>[2x]APSFNVDPLEQPAEPSKLAKKLRAEPDMDTSFVGLTGGQIFNEMMSRQNVDTVFGYPGGAILPVYDAIHNSDKFNFVLPKHEQGAGHMAEGYARASGKPGVVLVTSGPGATNVVTPMADAFADGIPMVVFTGQVPTSAIGTDAFQEADVVGISRSCTKWNVMVKSVEELPLRINEAFEIATSGRPGPVLVDLPKDVTAAILRNPIPTKTTLPSNALNQLTSRAQDEFVMQSINKAADLINLAKKPVLYVGAGILNHADGPRLLKELSDRAQIPVTTTLQGLGSFDQEDPKSLDMLGMHGCATANLAVQNADLIIAVGARFDDRVTGNISKFAPEARRAAAEGRGGIIHFEVSPKNINKVVQTQIAVEGDATTNLGKMMSKIFPVKERSEWFAQINKWKKEYPYAYMEETPGSKIKPQTVIKKLSKVAN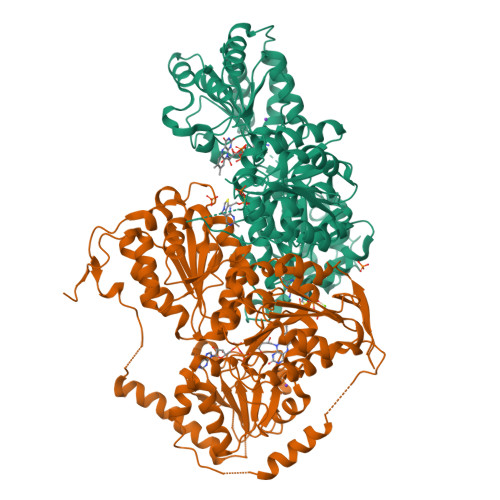DTGRHVIVTTGVGQHQMWAAQHWTWRNPHTFITSGGLGTMGYGLPAAIGAQVAKPESLVIDIDGDASFNMTLTELSSAVQAGTPVKILILNNEEQGMVTQWQSLFYEHRYSHTHQLNPDFIKLAEAMGLKGLRVKKQEELDAKLKEFVSTKGPVLLEVEVDKKVPVLPMVAGGSGLDEFINFDPEVERQQTELRHKRTGGKH> AAPAYGQPSAAMGQNMRPMNQLYPIDLLTELPPPITDLTLPPPPLVIPPERMLVPSELSNASPDYIRSTLNAVPKNSSLLKKSKLPFGLVIRPYQHLYDDIDPPPLNEDGLIVRCRRCRSYMNPFVTFIEQGRRWRCNFCRLANDVPMQMDQSDPNDPKSRYDRNEIKCAVMEYMAPKEYTLRQPPPATYCFLIDVSQSSIKSGLLATTINTLLQNLDSIPNHDERTRISILCVDNAIHYFKIPLDSENNEESADQINMMDIADLEEPFLPRPNSMVVSLKACRQNIETLLTKIPQIFQSNLITNFALGPALKSAYHLIGGVGGKIIVVSGTLPNLGIGKLQRRNESGVVNTSKETAQLLSCQDSFYKNFTIDCSKVQITVDLFLASEDYMDVASLSNLSRFTAGQTHFYPGFSGKNPNDIVKFSTEFAKHISMDFCMETVMRARGSTGLRMSRFYGHFFNRSSDLCAFSTMPRDQSYLFEVNVDESIMADYCYVQVAVLLSLNNSQRRIRIITLAMPTTESLAEVYASADQLAIASFYNSKAVEKALNSSLDDARVLINKSVQDILATYKKEIVVSNTAGGAPLRLCANLRMFPLLMHSLTKHMAFRSGIVPSDHRASALNNLESLPLKYLIKNIYPDVYSLHDMADEAGLPVQTEDGEATGTIVLPQPINATS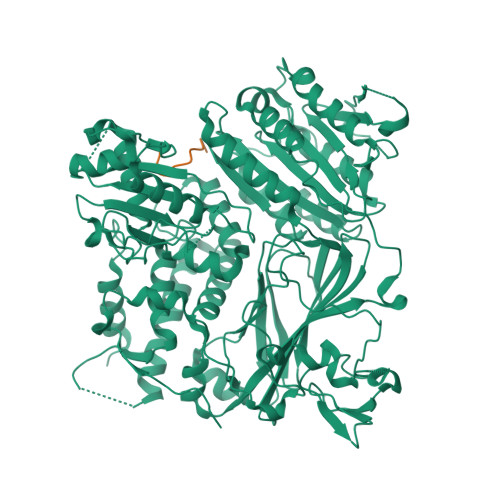SLFERYGLYLIDNGNELFLWMGGDAVPALVFDVFGTQDIFDIPIGKQEIPVVENSEFNQRVRNIINQLRNHDDVITYQSLYIVRGASLSEPVNHASAREVATLRLWASSTLVEDKILNNESYREFLQIMKARISK;> TYNNSNPFMT>GSVERVSLFPSYKLKIIQGNELEPRAVAALRPGMTKDQVLLLLGSPILRDAFHTDRWDYTFNTSRNGIIKERSNLTVYFENGVLVRTEGDALQNAAEALRAKQNADKQ[2x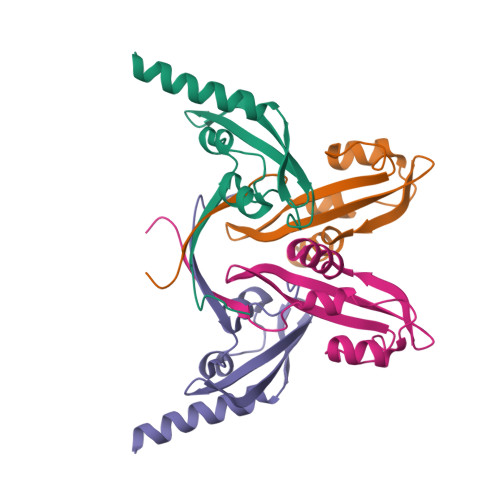]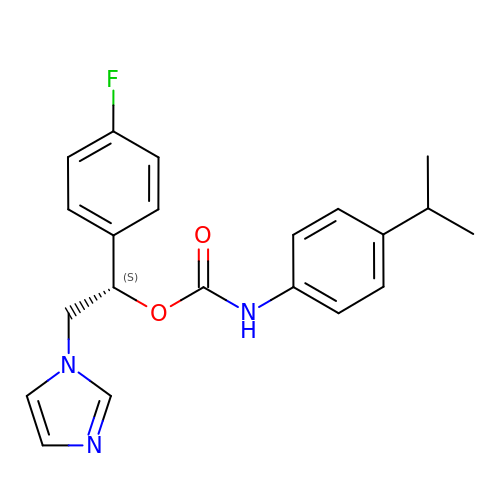(1S)-1-(4-fluorophenyl)-2-(1H-imidazol-1-yl)ethyl 4-isopropylphenylcarbamate | C21 H22 F N3 O2 | OMXCIRVMHPGVCD-HXUWFJFHSA-N> SAAGKDCITIHSATFAWSQESPPCLHRINLTVPQGCLLAV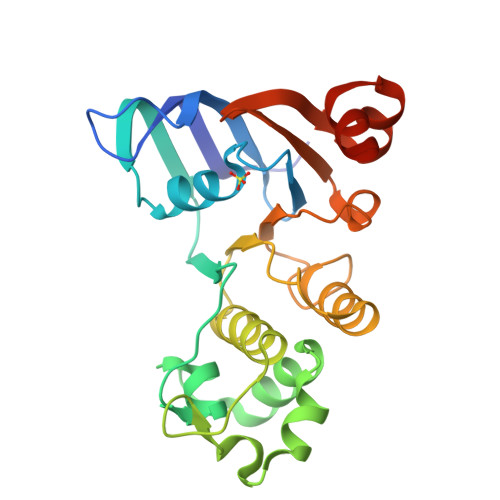VGPVGAGKSSLLSALLGELSKVEGFVSIEGAVAYVPQEAWVQNTSVVENVCFGQELDPPWLERVLEACALQPDVDSFPEGIHTSIGEQGMNLSGGQKQRLSLARAVYRKAAVYLLDDPLAALDAHVGQHVFNQVIGPGGLLQGTTRILVTHALHILPQADWIIVLANGAIAEMGSYQELLQRKGALVCLLDQARQPGD>[2x]RTFDLEEKLQTNKYNANFVTFMEGKDFNVEYIQRGGLRDPLIFKNSDGLGIKMPDPDFTVNDVKMCVGSRRM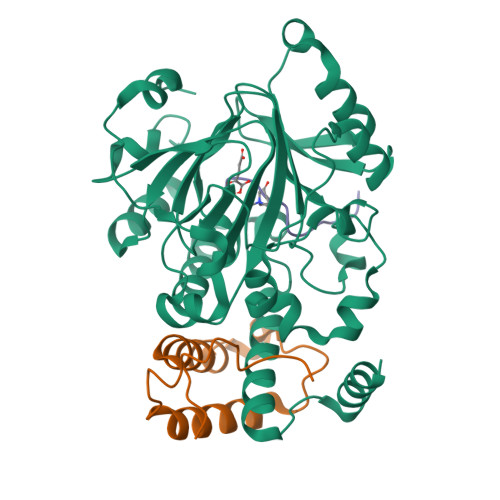VDVMDVNTQKGIEMTMAQWTRYYETPEEEREKLYNVISLEFSHTRLENMVQRPSTVDFIDWVDNMWPRHLKESQTESTNAILEMQYPKVQKYCLMSVRGCYTDFHVDFGGTSVWYHIHQGGKVFWLIPPTAHNLELYENWLLSGKQGDIFLGDRVSDCQRIELKQGYTFVIPSGWIHAVYTPTDTLVFGGNFLHSFNIPMQLKIYSIEDRTRVPNKFRYPFYYEMCWYVLERYVYCITNRSHLTKDFQKESLSMDME;>[2x]QVHLTHFELEGLRCLVDKLESLPLHKKCVPTGIEDEDALIADVKILLEELASSDPKLALTGVPIVQWP;>[2x]APATGGVKKPHRYRP>[2x]GSHMDRDIPLKGLLSIILRSHRVFIGRELGHLNLTDAQVACLLRIHREPGIKQDELATFFHVDKGTIARTLRRLEESGFIEREQDPENRRRYILEVTRRGEEIIPLILKVEERWEDLLF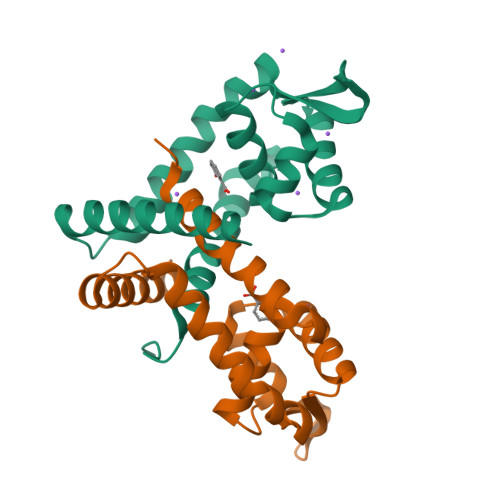RDFTEDERKLFRKMCRRLAEEAVRMRGEW>MTNAMKVEGYPSMEWPTSLDIPLKASEELVGIDLETDLPDDPTDLKTLLVEENSEKEHWLTIALAYCNHGKTNEGIKLIEMALDVFQNSERASLHTFLTWAHLNLAKGQSLSVETKEHELTQAELNLKDAIGFDPTWIGNMLATVELYYQRGHYDKALETSDLFVKSIHAEDHRSGRQSKPNCLFLLLRAKLLYQKKNYMASLKIFQELLVINPVLQPDPRIGIGLCFWQLKDSKMAIKSWQRALQLNPKNTSASILVLLGEFRESFTNSTNDKTFKEAFTKALSDLNNIFSENQHNPVLLTLLQTYYYFKGDYQTVLDIYHHRILKMSPMI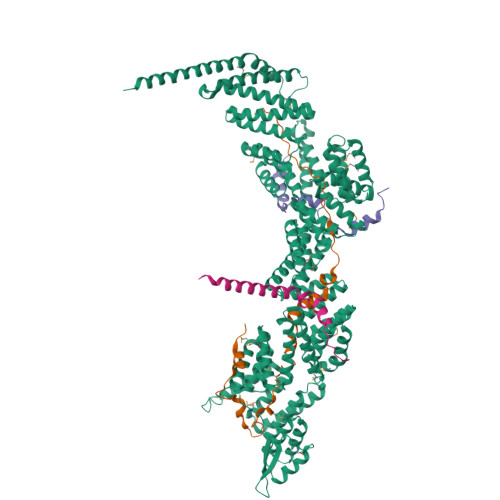AKIVLSESSFWCGRAHYALGDYRKSFIMFQESLKKNEDNLLAKLGLGQTQIKNNLLEESIITFENLYKTNESLQELNYILGMLYAGKAFDAKTAKNTSAKEQSNLNEKALKYLERYLKLTLATKNQLVISRAYLVISQLYELQNQYKTSLDYLSKALEEMEFIKKEIPLEVLNNLACYHFINGDFIKADDLFKQAKAKVSDKDESVNITLEYNIARTNEKNDCEKSESIYSQVTSLHPAYIAARIRNLYLKFAQSKIEDSDMSTEMNKLLDLNKSDLEIRSFYGWYLKNSKERKNNEKSTTHNKETLVKYNSHDAYALISLANLYVTIARDGKKSRNPKEQEKSKHSYLKAIQLYQKVLQVDPFNIFAAQGLAIIFAESKRLGPALEILRKVRDSLDNEDVQLNLAHCYLEMREYGKAIENYELVLKKFDNEKTRPHILNLLGRAWYARAIKERSVNFYQKALENAKTALDLFVKESSKSKFIHSVKFNIALLHFQIAETLRRSNPKFRTVQQIKDSLEGLKEGLELFRELNDLKEFNMIPKEELEQRIQLGETTMKSALERSLNEQEEFEKEQSAKIDEARKILEENELKEQGWMKQEEEARRLKLEKQAEEYRKLQDEAQKLIQEREAMAISEHNVKD[3x];>MSKKQEYIAPIKYQNSLPVPQLPPKLLVYPESPETNADSSQLINSLYIKTNVTNLIQQDEDLGMPVDLMKFPGLLNKLDSKLLYGFDNVKLDKDDRILLRDPR[3x];>NDSEVSDPVVVETMKHERILVDHNSALRGAKPINFGYLIKDAELKLVQSIKGSLRGS[3x];>[3x]KTRTKVYYQEIQKEENAKAKEIAQQEKLQEDKDAKDKREKELLVAQFRRLGGLERMVGELDIKFDLKF1-[2-methyl-1,3-bis(oxidanyl)propan-2-yl]-3-phenyl-urea 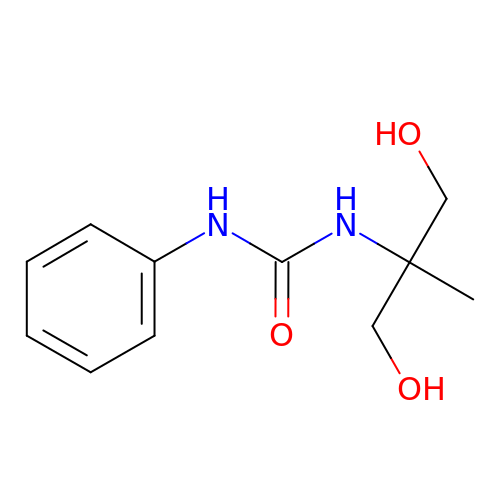| C11 H16 N2 O3 | NLGYHTMGWVQQIL-UHFFFAOYSA-N> MVSRIICFTLVLVTVVALSYGAAGRESSGGQKWRWGWDPLIRSPVDA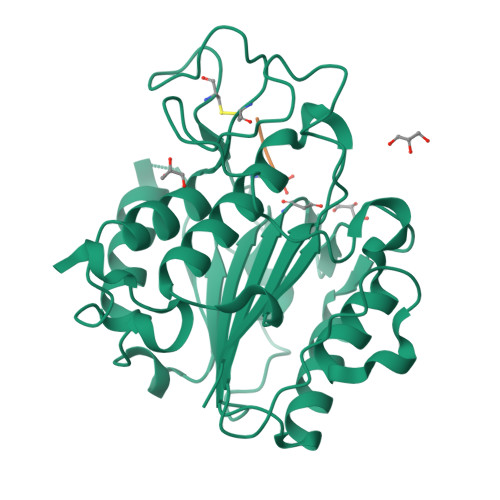EQEVDEQMTNGTKWAVLVAGSKGYGNYRHQADVCHAYQVLKKGGLKDENIVVFMYDDIAKSEMNPRPGIIINSPKGEDVYAGVPKDYTGKNVTVDNLSAVLLGDRSAVKGGSGKVVDSKPEDRIFLFYSNHGGPGVLGMPNEPHLVAKDLVDVLKKKHAMGTYKEMVIYLEACESGSIFEGILPEDLNIYATTASGAQENSYGTYCPGTEPSPPPEYITCLGDLYSVAWMEDSETHNLKKESLEQQFNKVKKRTSNSNTYNTGSHVMEYGSKDIKPEKVYLYLGFDPATVNLPANQIHFDKLDGVNQRDADLIFLWQRYKKSSESTRPEILREITETLTHRGHLDSSIDMIGVLLFGPQNGRSTLHSARAPGLPLVDDWECFKSTARLFEKHCGLLTQYGMKHMRAFANICNSSVEKSKVEEVFIATCGGKNIGPYGTFGAYSV> SDSAFSRYYT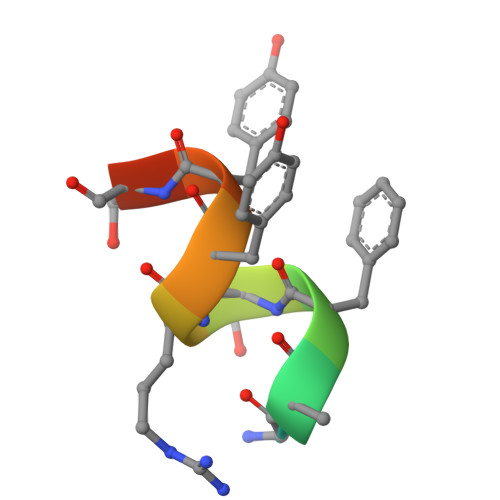RS>[2x]MGHHHHHHEFMTSRPSSDQTWQPIDGRVALIAPASAIATEVLEATLRQLEVHGVDYHLGRHVEARYRYLAGTVEQRL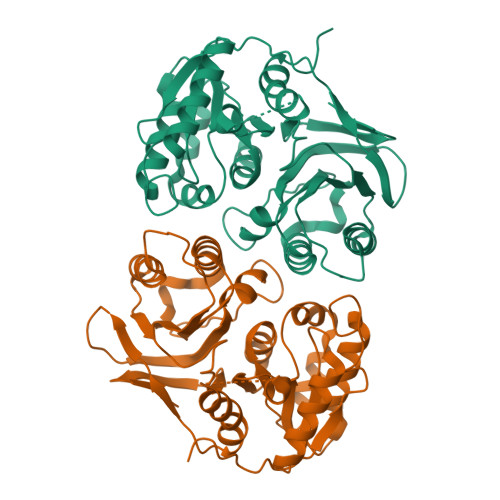EDLHNAFDMPDITAVWCLRGGYGCGQLLPGLDWGRLEAASPRPLIGFSDISVLLSAFHRHGLPAIHGPVATGLGLSPLSAPREQQERLASLASVSRLLAGIDHELPVQHLGGHKQRVEGALIGGNLTALACMAGTLGGLHAPAGSILVLEDVGEPYYRLERSLWQLLESIDARQLGAICLGSFTDCPRKEVAHSLERIFGEYAAAIEVPLYHHLPSGHGAQNRAWPYGKTAVLEGNRLRW> MGIMPRKVLAIKNFKERFDLLPKLKGVIAEKQPDILVVVGNILKNEALEKEYERAHLARREPNRKVIHENEHYIIETLDKFFREIGELGVKTFVVPGKNDAPLKIFLRAAYEAETAYPNIRVLHEGFAGWRGEFEVIGFGGLLTE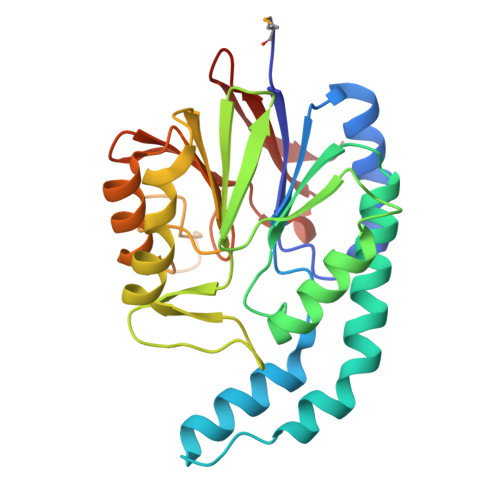HEFEEDFVLKYPRWYVEYILKFVNELKPRRLVTIFYTPPIGEFVDRTPEDPKHHGSAVVNTIIKSLNPEVAIVGHVGKGHELVGNTIVVNPGEFEEGRYAFLDLTQHKIKLEQFS>MAHHHHHHMADFNQILTPGDVDGGIINVVNEIPAGSNHKIEWNRKLAAFQLDRIEPAIF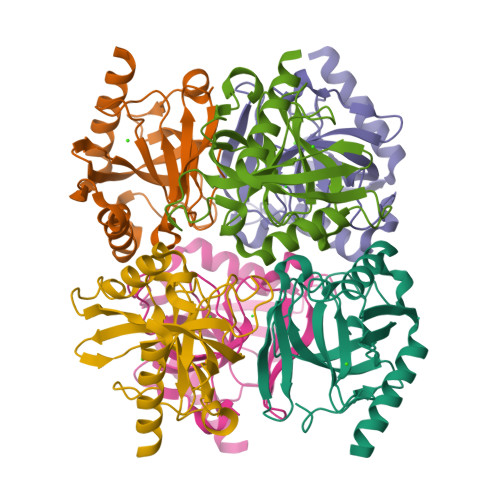AKPTNYGFIPQTLDEDGDELDVLLVTEQPLATGVFLEARVIGVMKFVDDGEVDDKIVCVPADDRNNGNAYKTLSDLPQQLIKQIEFHFNHYKDLKKAGTTKVESWGGAEEAKKVIKESIERWNKQA[6x]> SGAISGDSLISLASTGKRVSIKDLLDEKDFEIWAINEQTMKLESAKVSRVFMTGKKLVYILKTRLGRTIKATANHRFLTIDGWKRLDE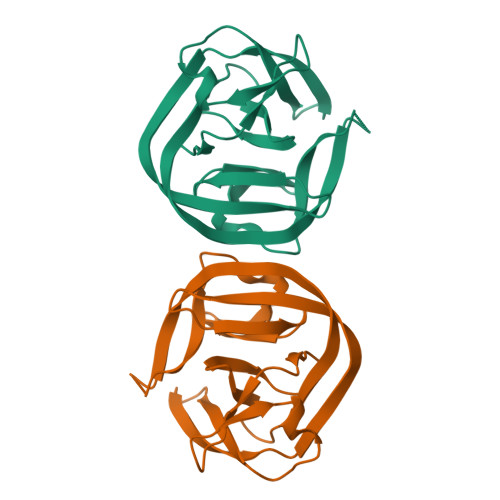LSLKEHIALPRKLESSSLQLSPEIEKLSQSDISWDSIVSITETGVEEVFDLTVPGPHNFVANDIIVHASI1,6-DIHYDROXY NAPHTHALENE | C10 H8 O2 | 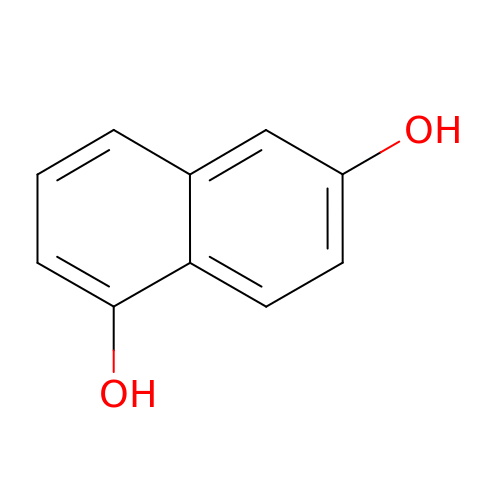FZZQNEVOYIYFPF-UHFFFAOYSA-N N-{4-[(4-ethylpiperazin-1-yl)methyl]-3-(trifluoromethyl)phenyl}-4-methyl-3-(1H-pyrrolo[2,3-b]pyridin-4-yloxy)benzamide | C29 H30 F3 N5 O2 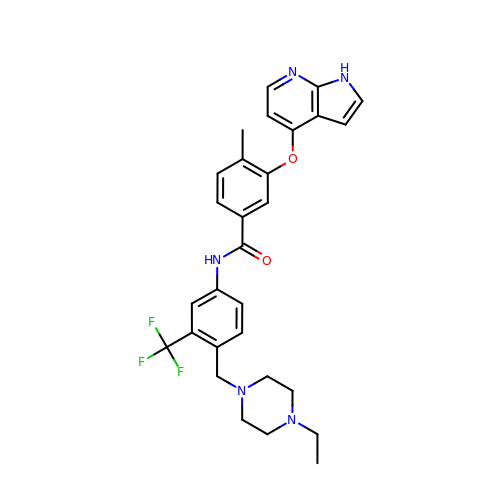| SMPGEBOIKULBCT-UHFFFAOYSA-N>[4x]WEEEDVICDGCNGPVVG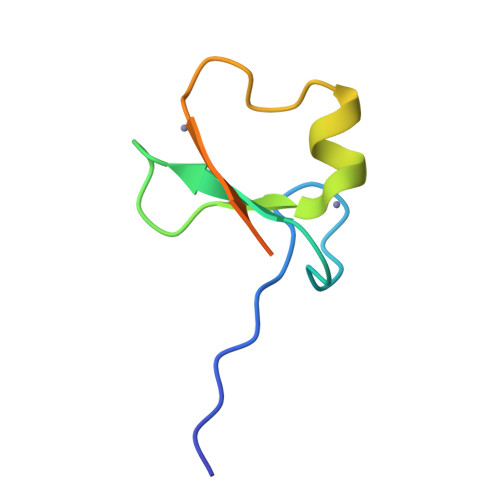TRYKCSVCPDYDLCSVCEGKGLHRGHTKLAFPSPFGHLSEGFS> MGNEFDKILKIIQKDIPLVKEPFSVLAQEVGIEEGKLLKTIEKLVEDGIVRHIAPIYDSRLLGYDSALIAFKVDRQKLEEVANFVNACPGVSHNYERTHDFNLWFT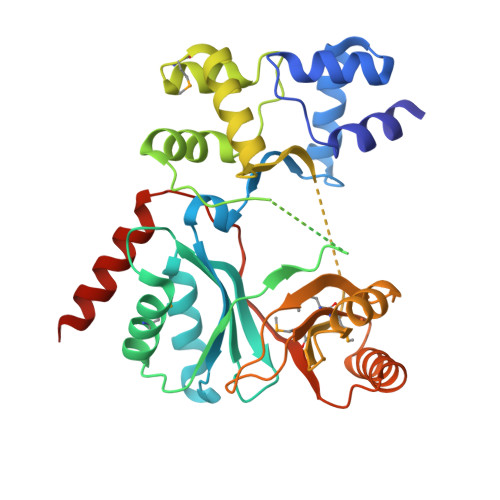LAVPPEISELEDVVRLMAERERVKDYLVLRVVRLFKIGVKLDYESPAEKESVDTKVYTYTPLTEEEKRIVSITQGSFPLVERPFLEYAKRLRMSEEELLEKLSALKERGVLRRISAVLYHRRAGYVANAMSVWEVPEDAIEEVGRYIAGFKGVSHCYQRTTSEKFRYNLFAMMHGKGQEEIKLLAETISREKALSKYALLFSTREFKKVRIKYFSEEFERWFKELISALEHHHHHH> MFENITAAPADPILGLADLFRADERPGKINLGIGVYKDETGKTPVLTSVKKAEQYLLENETTKNYLGIDGIPEFGRCTQELLFGKGSALINDKRARTAQTPGGTGALRVAADFLAKNTSVKRVWVSNPSWPNHKSVFNSAGLEVREYAYYDAENHTLDFDALINSLNEAQAGDVVLFHGCCHNPTGIDPTLEQWQTLAQLSVEKGWLPLFDFAYQGFARGLEEDAEGLRAFAAMHKELIVASSYSANFGLYNERVGACTLVAADSETVDRAFSQMKAAIRANYSNPPAHGASVV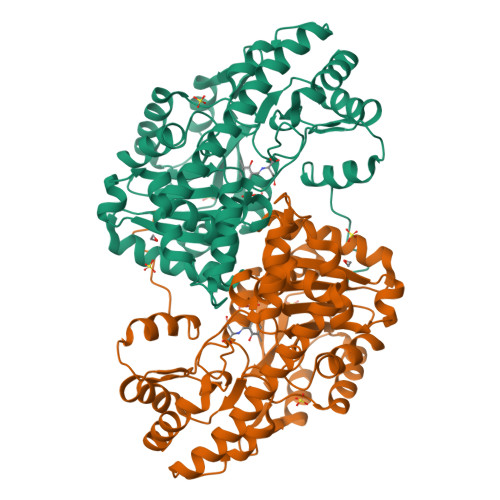ATILSNDALRAIWEQELTDMRQRIQRMRQLFVNTLQEKGANRDFSFIIKQNGMFSFSGLTKEQVLRLREEFGVYAVASGRVNVAGMTPDNMAPLCEAIVAVL> GMLED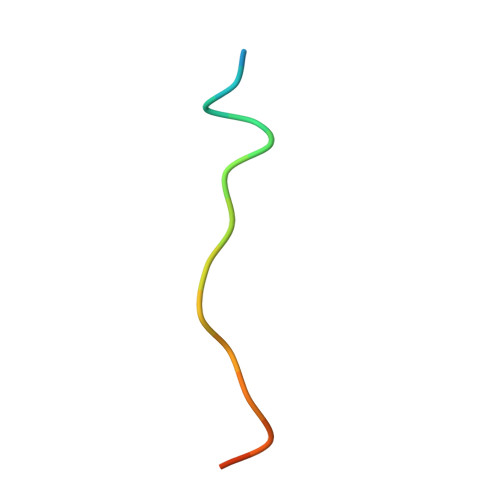LINSHADVNAVDD O6-CYCLOHEXYLMETHOXY-2-(4'-SULPHAMOYLANILINO) 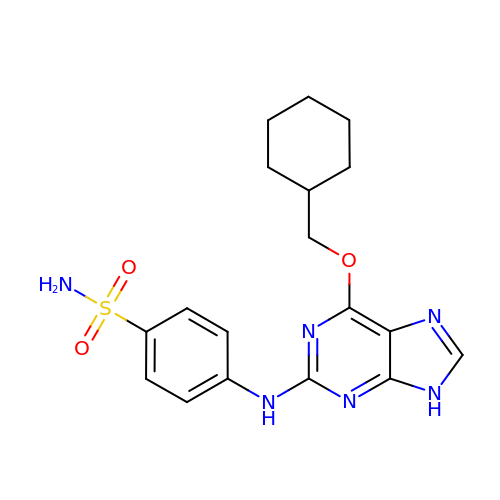PURINE | C18 H22 N6 O3 S | OWXORKPNCHJYOF-UHFFFAOYSA-N>[6x]SVIKPDMKIKLRMEGAVNGHPFAIEGVGLGKPFEGKQSMDLKVKEGGPLPF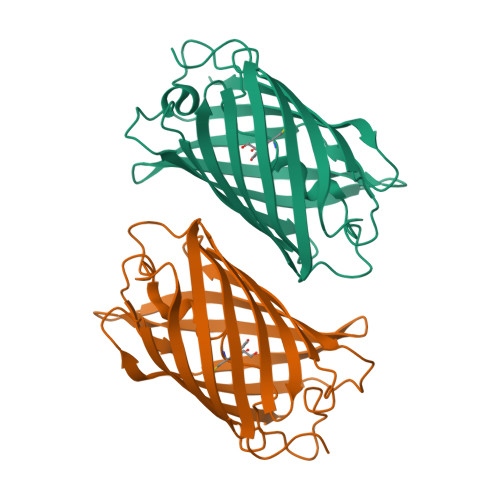AYDILTMAFCYGNRVFAKYPENIVDYFKQSFPEGYSWERSMIYEDGGICNATNDITLDGDCYIYEIRFDGVNFPANGPVMQKRTVKWELSTEKLYVRDGVLKSDGNYALSLEGGGHYRCDFKTTYKAKKVVQLPDYHSVDHHIEIKSHDKDYSNVNLHEHAEAHSE>MQLRSVIAADHPALFALWSRTPGIRL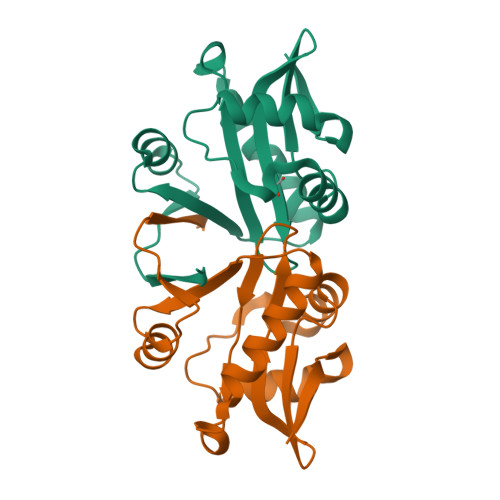RAEDAYPFFLAYLQRNPGLSLLVETEGEVIACLMAGHDGRRGYLQHLVVDPGYRGLGLARRMLDEVLARLAREGIGKSHVFVLDAAEEAQAFWRAQSDWERRKDIQVFSTREGHA[9x]> MKHHHHHHMKQNSPLDEENLTQENQDRGTHVDRGLASANVDFAFSLYKQLVLKAPDKNVIFSPLSISTALAFLSLGAHNTTLTEILKGLKFNLTETSEAEIHQSFQHLLRTLNQSSDELQLSMGNAMFVKEQLSLLDRFTEDAKRLYGSEAFATDFQDSAAAKKLINDYVKNGTRGKITDLIKDLDSQTMMVLVNYIFFKAKFEMPFDPQDTHQSRFYLSKKKYVMVPMMSLHHLTIPYFRDEELSCTVVQLNY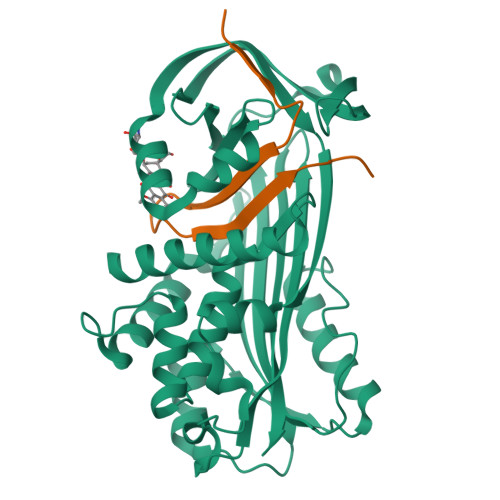TGNASALFILPDQDKMEEVEAMLSQETLSRFFESLEFREIGELYLPKFSISRDYNLNDILLQLGIEEAFTSKADLSGITGARNLAVSQVVHKAVLDVFEEGTEASAATALEVLFQ;> GPLVETRTIVRFNRPFLMIIVDNFTWSIFFMSKVTNPKQA> MDVVIAVGAPLTGPNAAFGAQIQKGAEQAAKDINAAGGINGEQIKIVLGDDVSDPKQGISVANKFVADGVKFVVGHFNSGVSIPASEVYAENGILEITPAATNPVFTERGLWNTFRTCGRDDQQGGIAGKYLADHFKDAKVAIIHDKTPYGQGLADETKKAANAAGVTEVMYEGVNVGDKDFSALISKMKEAGVSIIYWGGLHTEAGLIIRQAADQGLKAKLVSGDGIVSNELASIAGDAVEGTLNTFGPDPTLRPENKELVEKFKAAGFNPEAYTLYSYAAMQAIAGAAKAAGSVEP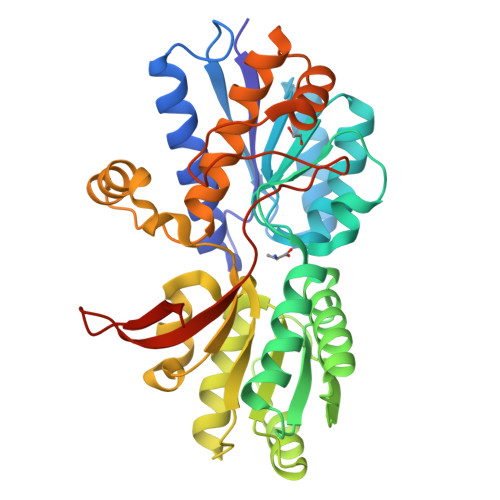EKVAEALKKGSFPTALGEISFDEKGDPKLPGYVMYEWKKGPDGKFTYIQQGSHHHHHH>MADTKAKLTLNGDTAVELDVLKGTLGQDVIDIRTLGSKGVFTFDPGFTSTASCESKITFIDGDEGILLHRGFPIDQLATDSNYLEVCYILLNGEKPTQEQYDEFKTTVTRHTMIHEQITRLFHAFRRDSHPMAVMCGITGALAAFYHDSLDVNNPRHREIAAFRLLSKMPTMAAMCYKYSIGQPFVYPRNDLSYAGNFLNMMFSTPCEPYEVNPILERAMDRILILHADHEQNASTSTVRTAGSSGANPFACIAAGIASLWGPAHGGANEAALKMLEEISSVKHIPEFFRRAKDKNDSFRLMGFGHRVYKNYDPRATVMRETCHEVLKELGTKDDLLEVAMELENIALNDPYFIEKKLYPNVDFYSGIILKAMGIPSSMFTVIAAMARTVGWI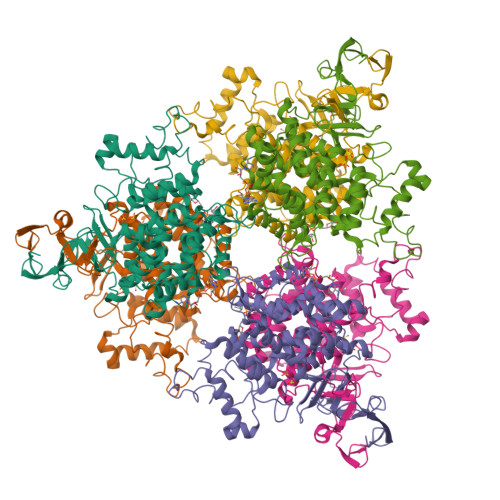AHWSEMHSDGMKIARPRQLYTGYEKRDFKSDIKR[2x]> MAQQRALPQSKETLLQSYNKRLKDDIKSIMDNFTEIIKTAKIEDETQVSRATQGEQDNYEMHVRAANIVRAGESLMKLVSDLKQFLILNDFPSVNEAIDQRNQQLRTLQEECDRKLITLRDEISID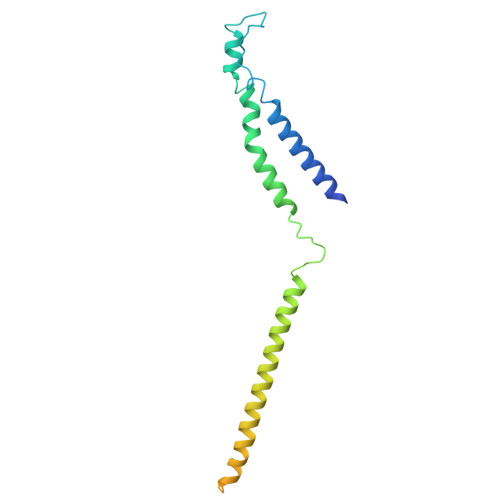LYELEEEYYSSSSSLCEANDLPLCEAYGRLDLDTDSADGLSAPLLASPEPSAGPLQVAAPAHSHAGGPGPTEHA> GPGSMKQYVARLEKDFSLIEHGFKEEEQRALTDYKSNDGEYIKKLAFLAYQSDVYQVRMYAVFLFGYLSKDKEILIFMRDEVSKDNNWRVQEVLAKAFDEFCKKIGYKKALPIIDEWLKSSNLHTRRAATEGLRIWTNRPYFKENPNEAIRRIADLKEDVSEYVRKSVGNALRDISKKFPDLVKIELKNWKLESKEINQVYKLASKFIDA

The HEAT-like repeat (HLR) DNA glycosylases exist in all domains of life and are structurally and mechanistically distinct from their base-flipping counterparts. These enzymes are composed of tandem helical HLR units that form an overall solenoid shape with a concave, positively charged DNA binding surface, and represent the first example of such an architecture to support DNA binding or catalytic activity. Here, we describe a new family of proteins related to the HLR DNA glycosylases that lacks DNA binding specificity as well as alkylpurine excision activity. We identified a fifth family, which we designate AlkD2, not present in B. cereus but spread across phylogenetically diverse bacteria, commonly in species which also possess AlkD.

Crystallographic analysis revealed that Streptococcus mutans AlkD2 is structurally similar to AlkD but lacks the DNA penetrating B-helix. We developed improved crystallization conditions that provided electron density for the missing parts of the search model, permitting a more complete and detailed structural analysis. In SmAlkD2, the N-terminal capping motif lacks helix B, and helices A and C are instead connected by a short loop. The loss of helix B is accompanied by a ~10 Å translation of helix C toward helix E. The positions of the corresponding residues in the sequence alignment suggest that helix C is also rotated by 180° about its longitudinal axis. These spatial differences would eliminate or alter interactions between helix C of BcAlkD and DNA. Of the five DNA binding residues located in the ABC motif of BcAlkD, only one is appropriately positioned to interact with DNA in the A−C motif of SmAlkD2. The position of a bound phosphate ion in the SmAlkD2 structure, however, suggests that SmAlkD2 may interact with DNA through two residues, His17 and Arg85, not shared with BcAlkD. Interestingly, SmAlkD2 retains a largely positively charged concave surface despite its low sequence similarity to AlkD. Conversely, SmAlkD2 failed to increase the amounts of 3mA and 7mG relative to a buffer-only control. In contrast, SmAlkD2 bound G•T-DNA with the same low-micromolar affinity as G•C-DNA and bound THF•C-DNA only 20-fold more tightly.> EDGKPVWAPHPTDGFQVGNIVDIGPDSLTIEPLNQKGKTFLALINQVFPAEEDSKKDVEDNCSLMYLNEATLLHNIKVRYSKDRIYTYVANI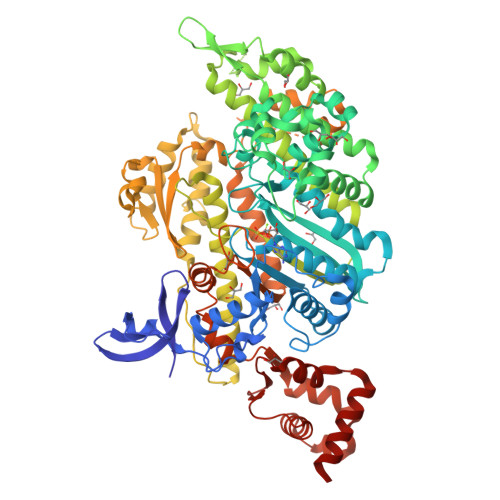LIAVNPYFDIPKIYSSETIKSYQGKSLGTMPPHVFAIADKAFRDMKVLKLSQSIIVSGESGAGKTENTKFVLRYLTESYGTGQDIDDRIVEANPLLEAFGNAKTVRNNNSSRFGKFVEIHFNEKSSVVGGFVSHYLLEKSRICVQGKEERNYHIFYRLCAGASEDIRERLHLSSPDNFRYLNRGCTRYFANKETDKQILQNRKSPEYLKAGSLKDPLLDDHGDFIRMCTAMKKIGLDDEEKLDLFRVVAGVLHLGNIDFEEAGSTSGGCNLKNKSTQALEYCAELLGLDQDDLRVSLTTRVMLTTAGGAKGTVIKVPLKVEQANNARDALAKTVYSHLFDHVVNRVNQCFPFETSSYFIGVLDIEGFEYFEHNSFEQFCINYCNEKLQQFFNERILKEEQELYQKEGLGVNEVHYVDNQDCIDLIEARLVGILDILDEENRLPQPSDQHFTSAVHQKHKDHFRLSIPRKSKLAIHRNIRDDEGFIIRHFAGAVCYETTQFVEKNNDALHMSLESLICESRDKFIRELFESSTNNNKDTKQKAGKLSFISVGNKFKTQLNLLLDKLRSTGASFIRCIKPNLKMTSHHFEGAQILSQLQCSGMVSVLDLMQGGFPSRASFHELYNMYKKYMPDKLARLDPRLFCKALFKALGLNEIDYKFGLTKVFFRPGKFAEFDQIMKSDPDHLAELVKRVNHWLI8-OXODEOXYADENOSINE | C10 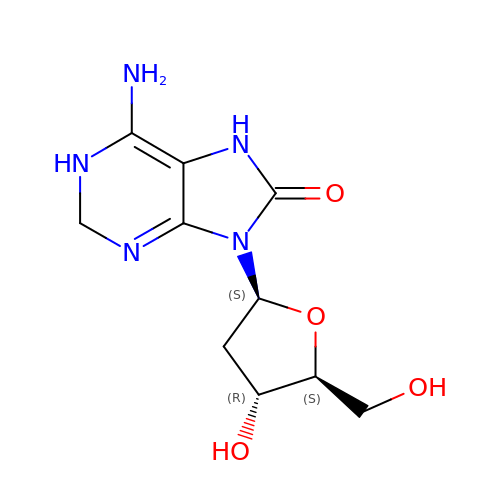H15 N5 O4 | KTCVXRUKSBTHOG-SRQIZXRXSA-N> GSHMATPP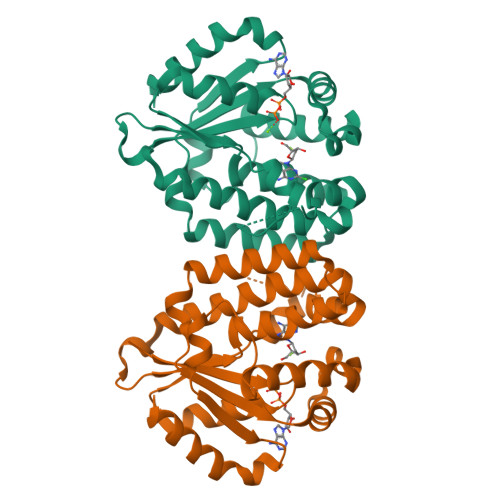KRSCPSFSASSEGTRIKKISIEGNIAAGKSTFVNILKQLCEDWEVVPEPVARWCNVQSTQDEFEELTMSQKNGGNVLQMMYEKPERWSFTFQTYACLSRIRAQLASLNGKLKDAEKPVLFFERSVYSDRYIFASNLYESECMNETEWTIYQDWHDWMNNQFGQSLELDGIIYLQATPETCLHRIYLRGRNEEQGIPLEYLEKLHYKHESWLLHRTLKTNFDYLQEVPILTLDVNEDFKDKYESLVEKVKEFLSTL>[4x]MKTVTVKNLIIGEGMPKIIVSLMGRDINSVKAEALAYREATFDILEWRVDH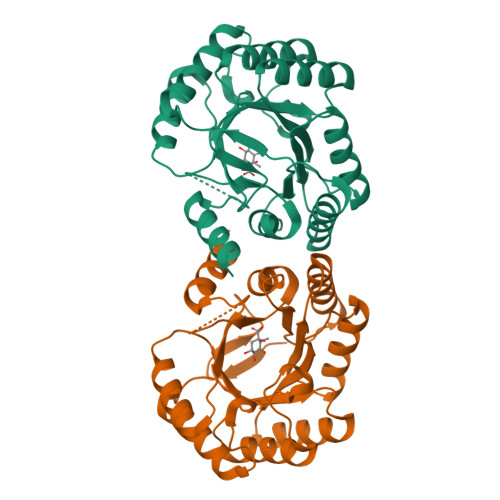FMDIASTQSVLTAARVIRDAMPDIPLLFTFRSAKEGGEQTITTQHYLTLNRAAIDSGLVDMIDLELFTGDADVKATVDYAHAHNVYVVMSNHDFHQTPSAEEMVLRLRKMQALGADIPKIAVMPQSKHDVLTLLTATLEMQQHYADRPVITMSMAKEGVISRLAGEVFGSAATFGAVKQASAPGQIAVNDLRSVLMILHNA(1S,3S,4S)-3-[(E)-({3-hydroxy-2-methyl-5-[(phosphonooxy)methyl]pyridin-4-yl}methylidene)amino]-4-(1,1,3,3,3-pentafluoroprop-1-en-2-yl)cyclopentane-1-carboxylic 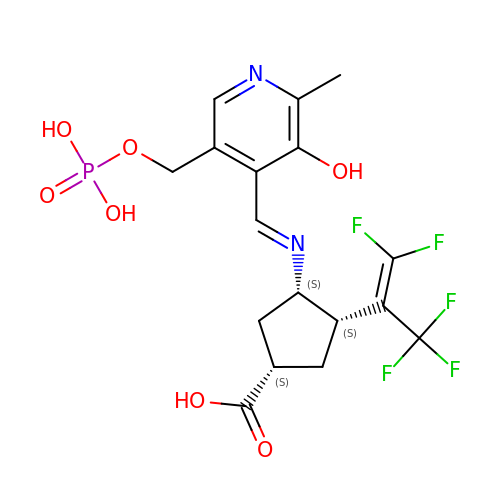acid | C17 H18 F5 N2 O7 P | NXIZEOJYEPCEAL-UJKLFKHKSA-N>[4x]MGSLTNHTETITVEEGQTLTLKCVTSLRKNSSL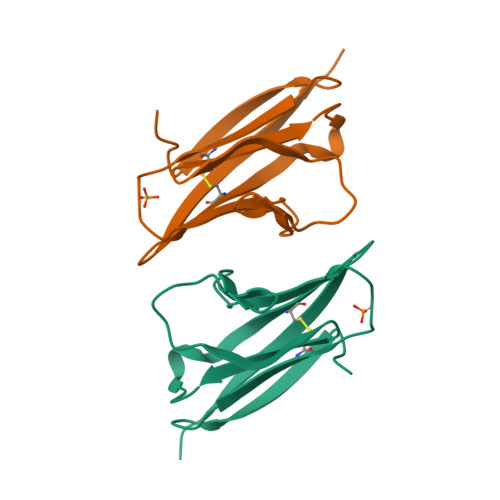QWLTPSGFTIFLNEYPVLKNSKYQLLHHSANQLSITVPNVTLQDEGVYKCLHYSDSVSTKEVKVIVLATMKGEFCRYPSHWRPLEHHHHHH> MAGKKRRLS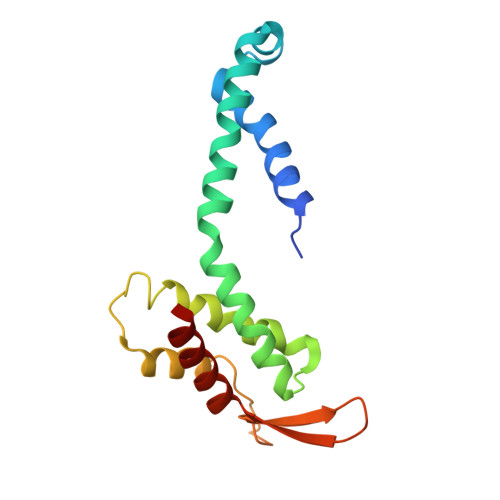QASVLRYYAKRFTMNVGTTAHVLGKEVAGNPWVAKAIDKLSYQETYNWISDYQASHLAKQVAKQVAEKYGIPPTFQGLLMAYAEKVVANYILDYKGESLTQMHDNYLYELMQKMPIAPTGTSSGYIYVFIGKDGKTHTVDMSKVLTDIEDALLKRA>[8x]DKLTLWTTLDPSPNCRIDVDKDSKLTLVLTKCGSQILANVSLLVVKGRFQNLNYKTNPNLPKTFTIKLLFDENGILKDSSNLDKNYWNYRNGNSILAEQY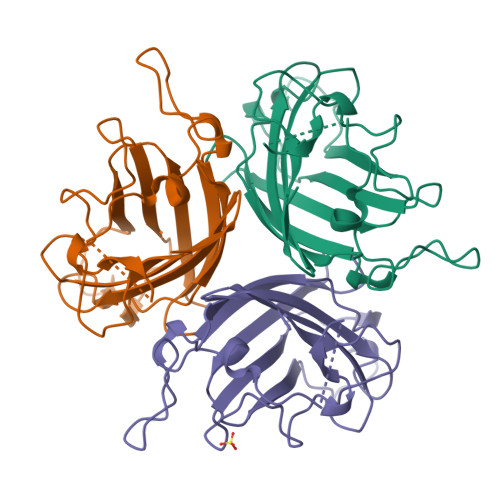KNAVGFMPNLAAYPKSTTTQSKLYARNTIFGNIYLDSQAYNPVVIKITFNQEADSAYSITLNYSWGKDYENIPFDSTSFTFSYIAQE> GAMGSGTARYHTQMLRVREFIRFHQIPNPLRQRLEEYFQHAWTYTNGIDMNSVLKGFPECLQADICLHLNRNLLNNCSAFEAASPGCLRALSLKFKTTHAPPGDILVHKGDVLTYLYFIARGSIEILKDDVVMAILGKDD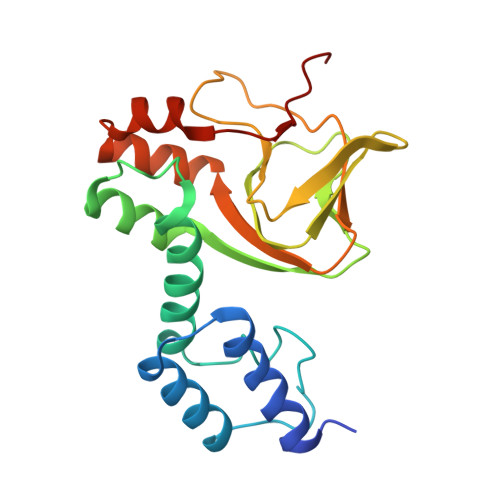IFGENPCIHSTLGKSNSNVKALTYCDLHKIHRDDLLDVLDLFPEFYDSFVNSLEITYNMRDEEQ> MHHHHHHFPEENIIDAKTRNEQTTI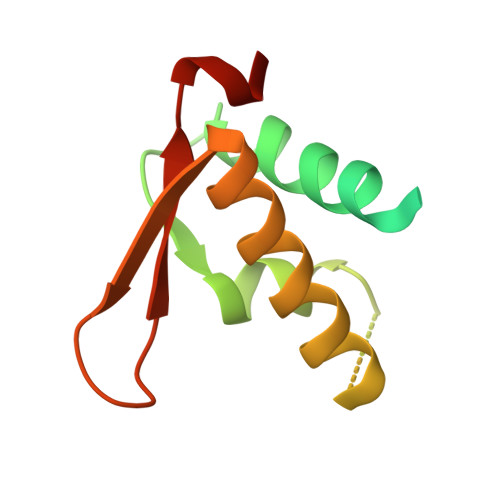QTEKVRPTPGEVASKAIVQMAKILRKELSEEKEVIFTDVLKSQANTEPENITKREASRGFFDILSLATEGCIGLSQTEAFGNIKIDAKPALFERFI> VKMSEEEEDLISRMYK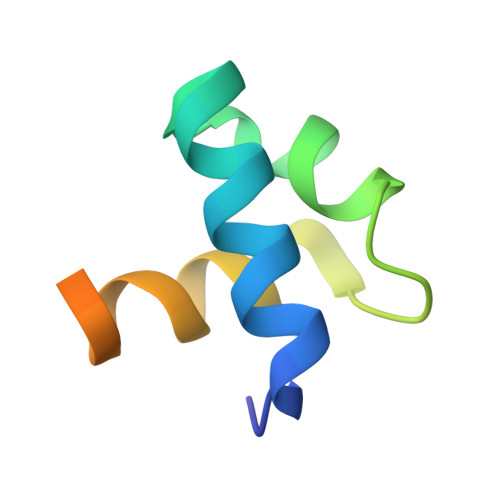LVGDRWELIAGRIPGRTPEEIERYWLMKHGVVFANRRRDFFRK The FPC is a macromolecular cytoskeletal structure and is essential for the formation of the FP and cytokinesis. Here, we report by yeast two-hybrid, bioinformatics, functional and structural studies the characterization of a new FPC component and BILBO1 partner protein, BILBO2 (Tb927.6.3240). Further, we demonstrate that BILBO1 and BILBO2 share a homologous NTD and that both domains interact with FPC4. We show that BILBO2 interacts with the BILBO1 EF-hand domains via its C-terminal domain and with FPC4 via its N-terminal domain. Together with BILBO1, BILBO2 is the second bona fide FPC protein and is involved in a tripartite interaction with BILBO1 and FPC4.

The crystal structure was determined at 1.86 Å resolution by molecular replacement using the structure of BILBO1-NTD (6JSQ.pdb) as the search model. There are two copies of the heterodimer per asymmetric unit in the crystal. Both structures contain aa4-110 of BILBO2 and aa432-438 of FPC4, except aa26-27 that were missing in one BILBO2 molecule. The two structures of the complex are nearly identical, with a root-mean-square deviation (RMSD) of 0.46 Å for all aligned backbone atoms. These two structures of BILBO2-NTD are also very similar to our previously reported crystal structure of BILBO1-NTD, with RMSD values of 0.84 Å and 0.98 Å. Similar to the BILBO1-NTD structure, the C-terminal part of BILBO2-NTD (aa91-110) also forms a horseshoe-like loop that wraps around the first two β strands and the long α helix of the core structure. FPC4 is docked into the hydrophobic cleft between the C-terminal loop and the β sheet. Interestingly, despite the fact that we used aa394-444 of FPC4 to prepare the sample for crystallization, only residues L432-P438 were visible in the final structure, suggesting that the rest of FPC4 does not bind to BILBO2 and is thus disordered as predicted. This part of FPC4, particularly residues S435 and P436 in the centre of the stretch, makes extensive contacts with BILBO2 through multiple hydrogen bonds and many hydrophobic interactions. The crystal structure of the BILBO2-FPC4 protein complex also suggests that residues F63, F88, and W70 in the BILBO2-NTD are involved in the interaction with FPC4.

>[2x]HMMGGISICVATDCDGEKVNLRFLFDAAGPSVSRLLNYSTTAFNNYFRLKGISRAFAVNSAVVFNDVHCTWDRLERTTQLLHNSQVYLFQPDTLDIPAAIPEPYEGEPLLSA;>SSLSPYLRYLPSDVSGGEWDKPDVGDVLCFQAKEPQRRRVLTSPVPDELLIK[2x]>MGTFTLHQGQTNLIKSFFRNYYLNAELELPKDMELREFALQPFGSDTYVRHLSFSSSEELRDYLVNRNLPLHLFYSSARYQLPSARNMEEKAWMGSDLLFDIDADHLCKLRSIRFCPVCGNAVVSEKCERDNVETLEYVEMTSECIKRGLEQTRNLVEILEDDFGLKPKVYFSGNRGFHVQVDCYGNCALLDSDERKEIAEYVMGIGVPGYPGGSENAPGWVGRKNRGINGVTIDEQVTIDVKRLIRIPNSLHGKSGLIVKRVPNLDDFEFNETLSPFTGYTIFLPYITIETEVLGSIIKLNRGIPIKIKSSIGIYLHLRNLGEVKAYVR[2x];>MALDVKKYPFIKSLDDELKKYGGGITLTDLLLNSTTLIDQAKDRIQKTKSGDELPHYVSYNEPVLVFYTTLLSLAILNDVKLIRRYAYAEAKQFRSLLHTENEENLLEISKLLDLKINRCDPIKFYLEKKRRIIQKEFCVHFIDYLKYTKDLKEDWKLSGQILHKGYVYLDKNQLIGLIAESIKSKIVEMIRPLNLKEIPEKLKSLIERRGIIPPCIENILAKEKLNEEEIRTLITFYIDIGKG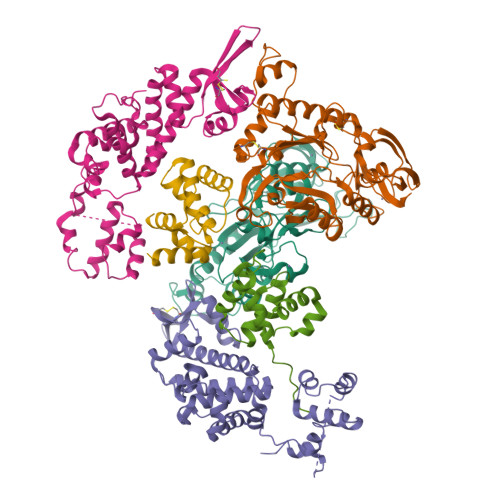LSGIVSIMKKYNVSNVEDLYRKYRGDKGTRYIVYSCAKMKQLGLCVSSCNVKNPLQLYFLSNE[2x];>[2x]MSQEKKAKKIILHYPDDTPAGYIEYAEGSSSIYDNEGNFLFKVEGKFPPQPKKSSDYSWIEKVLEMGLQDSRKRFILYVASRYLVNVKGVNEDEALQTLKEFYYKLQSGKVYESWLKSVINGVKKKGLLPWSLKRIEERDKEMYNEIIRVLKNS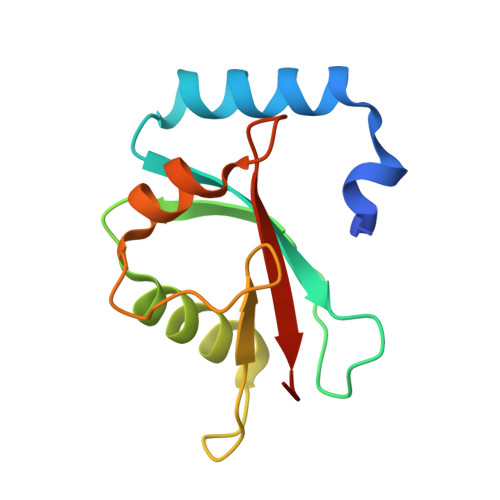> GPHMRSQFKDDFSFEKRKTESQRIREKYPDRIPVICEKVDKSDIAAIDKKKYLVPSDLTVGQFVYVIRKRIKLSPEKAIFIFIDEILPPTAALMSTIYEEHKSEDGFLYITYSGENTFG>ARKCSLTGKWTNDLGSNMTIGAVNSRGEFTGTYTTAVTATSNEIKESPLHGTENTINKRTQPTFGFTVNWKFSESTTVFTGQCFIDRNGKEVLKTMWLLRSSVNDIGD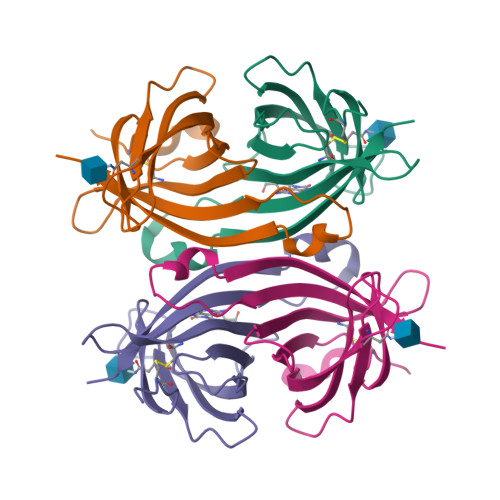DWKATRVGINIFTRLR[2x]N-(5-CHLORO-1,3-BENZODIOXOL-4-YL)-7-[2-(4-METHYLPIPERAZIN-1-YL)ETHOXY]-5-(TETRAHYDRO-2H-PYRAN-4-YLOXY)QUINAZOLIN-4-AMINE | C27 H32 Cl N5 O5 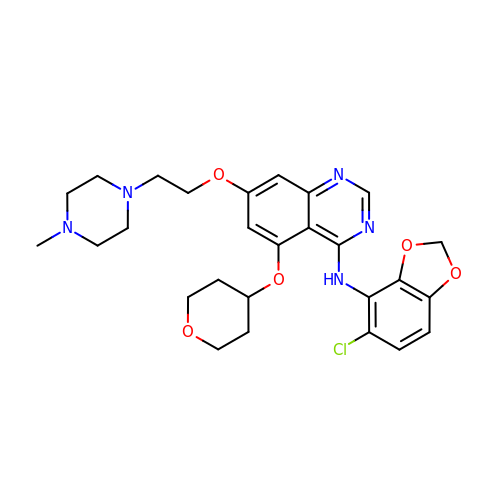| OUKYUETWWIPKQR-UHFFFAOYSA-N>MSASAETVAPEGYRKLLDVQIFKDSPVVGWSGSGMGELETIGDTLPVDTTVTYNGLPTLRLNVQTTVQSGWWISLLTLRGWNTHDLSQYVENGYLEFDIKGKEGGEDFVIGFRDKVYERVYGLEIDVTTVISNYVTVTTDWQHVKIPLRDLMKINNGFDPSSVTCLVFSKRYADPFTVWFSDIKITSEDNEKSAPAIKLEHHHHHH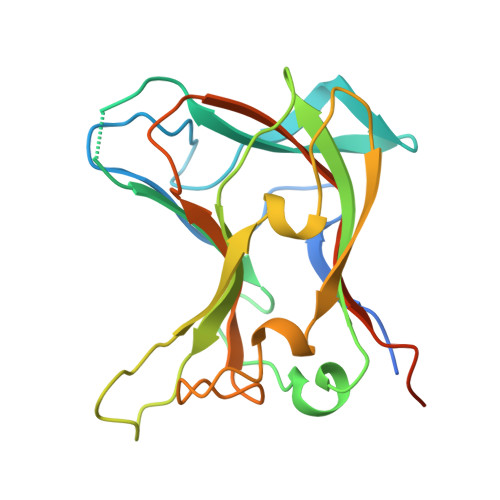[2x]> MLKQVEIFTDGSCLGNPGPGGYGAILRYR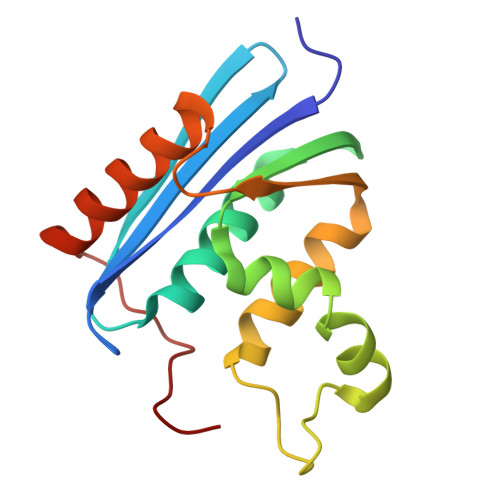GREKTFSAGYTRTTNNRMQLMAAIVALEALKEHCEVILSTDSQYVRQGITQWIHNWKKRGWKTADKKPVKNVDLWQRLDAALGQHQIKWEWVKGHAGHPENERCDELARAAAMNPTLEDTGYQVEV>[2x]MAADFETSNRRWLDKLPRNLTDSARSLHPRTLVAAIVVGLITGVLGAGFKSAVNNML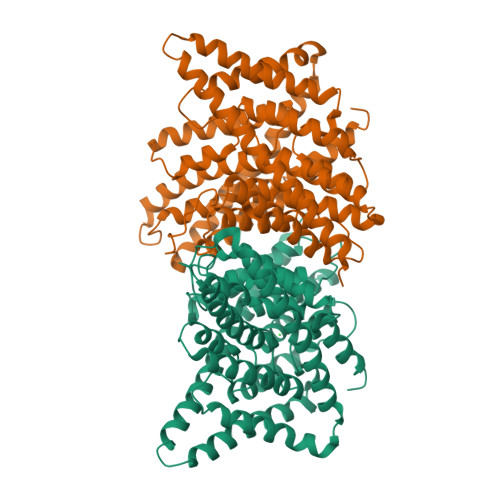QWRSQLAQILAPIPPLAWLVTALISGGMVALSFWLMKRFAPDTSGSGIPQIEGHLEGKLPLVWQRVLPIKLVGGFLSLGAGMLAGFEGPTIQMGGSIGQMTGGWFKATQENQRILIAVGAGAGLATAFNAPLAGVALIGEEMHPRFRSQTLAYHSLLFGCVMATIILRMIRGQSAIISLTEFKRVPLDSLWMFIILGILFGVMGYTFNRGLFKVLDWFDRLPPLATKWKGFLLGSIIGILSLFPLPLTDGGDNAVLWAFNSQSHFSTLILVFCGRFLLTLICYGSGAIGGIFAPMLGIASIVSVAMARHFHLLFPSQIPEPAVMAIAGMGALVAATVRAPLTAILLTIEMTDNYFVILPLLVTCLVASVVAEALGGKPIYTVLLERTLAKQNRGSLVPRGSGGHHHHHH(2~{S})-3-[4-[[5-(aminomethyl)furan-3-yl]methoxy]phenyl]-2-(methylamino)propanoic 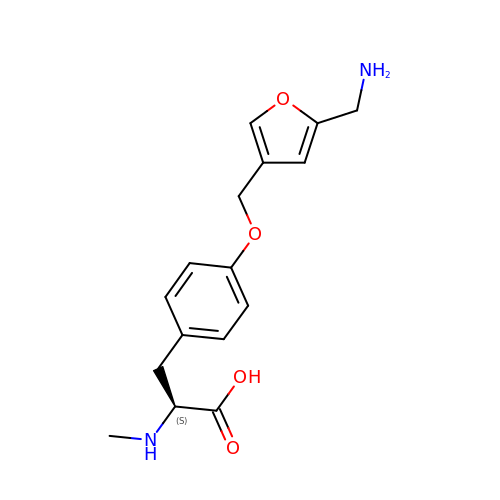acid | C16 H20 N2 O4 | QGZKJFPEUIZHQR-HNNXBMFYSA-N> MLESNENRIQIMSTIAKIYRAMSRELNRRLGELNLSYLDFLVLRATSDGPKTMAYLANRYFVTQSA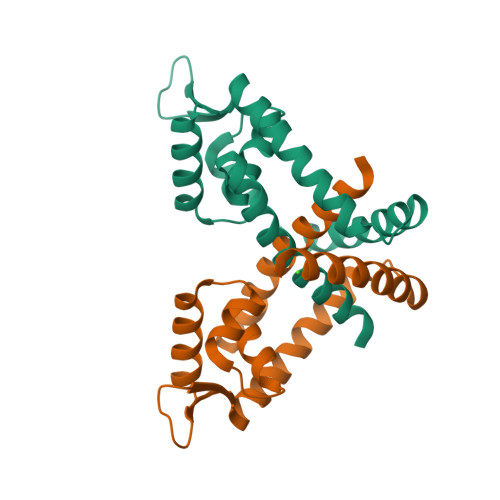ITASVDKLEEMGLVVRVRDREDARKILIEITEKGLETFNKGIEIYKKLANEVTGDLSEDEVILVLDKISKILKRIEEISQ> MKVGIDAGGTLIKIVQEQDNQRTFK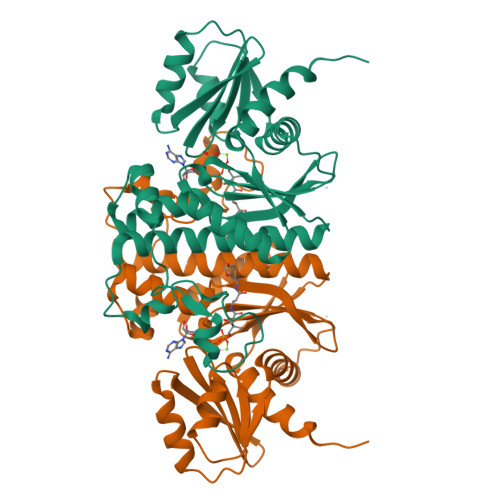TELTKNIDQVVEWLNQQQIEKLCLTGGNAGVIAENINIPAQIFVEFDAASQGLGILLKEQGHDLADYIFANVGTGTSLHYFDGQSQRRVGGIGTGGGMIQGLGYLLSQITDYKQLTDMAQHGDRNTIDLKVRHIYKDTEPPIPGDLTAANFGHVLHHLDADFTPSNKLAAVIGVVGEVVTTMAITVAREFKTENIVYIGSSFHNNALLRKVVEDYTVLRGCKPYYVENGAFSGAIGALYLEKHHHHHH> MELTPREKDKLLLFTAALVAERRLARGLKLNYPESVALISAFIMEGARDGKSVASLMEEGRHVLTREQVM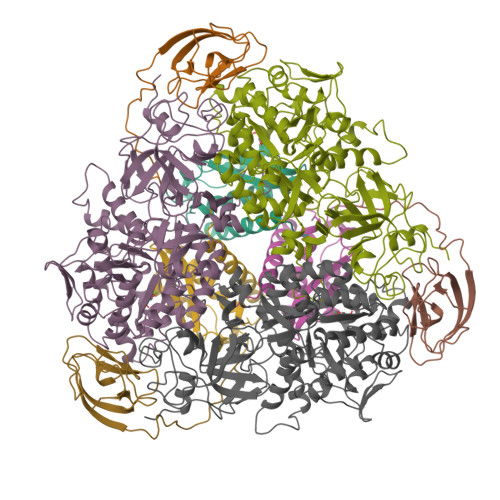EGVPEMIPDIQVEATFPDGSKLVTVHNPII;> MIPGEYHVKPGQIALNTGRATCRVVVENHGDRPIQVGSHYHFAEVNPALKFDRQQAAGYRLNIPAGTAVRFEPGQKREVELVAFAGHRAVFGFRGEVMGPLEVNDE;> MSNISRQAYADMFGPTVGDKVRLADTELWIEVEDDLTTYGEEVKFGGGKVIRDGMGQGQMLAADCVDLVLTNALIVDHWGIVKADIGVKDGRIFAIGKAGNPDIQPNVTIPIGAATEVIAAEGKIVTAGGIDTHIHWICPQQAEEALVSGVTTMVGGGTGPAAGTHATTCTPGPWYISRMLQAADSLPVNIGLLGKGNVSQPDALREQVAAGVIGLKIHEDWGATPAAIDCALTVADEMDIQVALHSDTLNESGFVEDTLAAIGGRTIHTFHTEGAGGGHAPDIITACAHPNILPSSTNPTLPYTLNTIDEHLDMLMVYHHLDPDIAEDVAFAESRIRRETIAAEDVLHDLGAFSLTSSDSQAMGRVGEVILRTWQVAHRMKVQRGALAEETGDNDNFRVKRYIAKYTINPALTHGIAHEVGSIEVGKLADLVVWSPAFFGVKPATVIKGGMIAIAPMGDINASIPTPQPVHYRPMFGALGSARHHCRLTFLSQAAAANGVAERLNLRSAIAVVKGCRTVQKADMVHNSLQPNITVDAQTYEVRVDGELITSEPADVLPMAQRYFLF> MAHHHHHHAEELVLERCDLE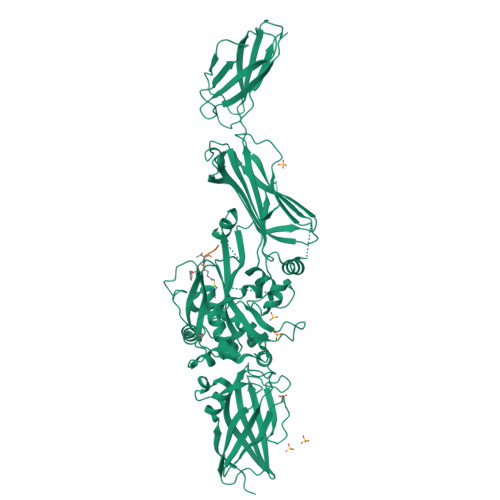LETNGRDHHTADLCREKLVVRRGQPFWLTLHFEGRNYEASVDSLTFSVVTGPAPSQEAGTKARFPLRDAVEEGDWTATVVDQQDCTLSLQLTTPANAPIGLYRLSLEASTGYQGSSFVLGHFILLFNAWCPADAVYLDSEEERQEYVLTQQGFIYQGSAKFIKNIPWNFGQFEDGILDICLILLDVNPKFLKNAGRDCSRRSSPVYVGRVVSGMVNCNDDQGVLLGRWDNNYGDGVSPMSWIGSVDILRRWKNHGCQRVKYGQCWVFAAVACTVLRCLGIPTRVVTNYNSAHDQNSNLLIEYFRNEFGEIQGDKSEMIWNFHCWVESWMTRPDLQPGYEGWQALDPTPQEKSEGTYCCGPVPVRAIKEGDLSTKYDAPFVFAEVNADVVDWIQQDDGSVHKSINRSLIVGLKISTKSVGRDEREDITHTYKYPEGSSEEREAFTRANHLNKLAEKEETGMAMRIRVGQSMNMGSDFDVFAHITNNTAEEYVCRLLLCARTVSYNGILGPECGTKYLLNLNLEPFSEKSVPLCILYEKYRDCLTESNLIKVRALLVEPVINSYLLAERDLYLENPEIKIRILGEPKQKRKLVAEVSLQNPLPVALEGCTFTVEGAGLTEEQKTVEIPDPVEAGEEVKVRMDLLPLHMGLHKLVVNFESDKLKAVKGFRNVIIGPA> MASEDKFESVLSTRYCKNSPLVSILSETNKATLWRQLWIWLAEAEKELGLKQVTQDAIDEMKSNRDVFDWPFIRSEERKLKHDVMAHNHAFGKLCPTAAGIIHLGATSCFVQDNADLIAYRDSIDHILKRFATVIDRLAAFSLKNKEVVTVGRTHYQTASLVTVGKRGVLWAQELLMAFQSLSEFRDKMRFRGIKGATGTQDSFLTLFAGDESKVEALDELVTKKANFSNRFLITGQTYSRQQDSQLVFSLSLLGAAA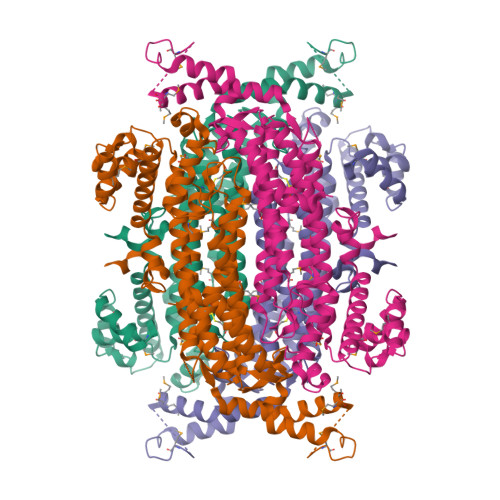KKVCTDIRVLQAFGELLEPFEKDQIGSSAMPYKKNPMKSERCCALSRKLINAPQEALTILADQGLERTLDDSAGRRMLIPDVLLTAEALLTTLQNIFEGLSVQTDNVKKIVEDEIAFLGLEKAMMMLTEEGVDRQQAHAVIRKTALEAKQLQATQKVDIRQTMADPFFDSVRDRVVGLVNNPINFTGRCVSQTESFIAKELKPTIDKYLDKSAGNVQLDV> EEASSTGRNFNVE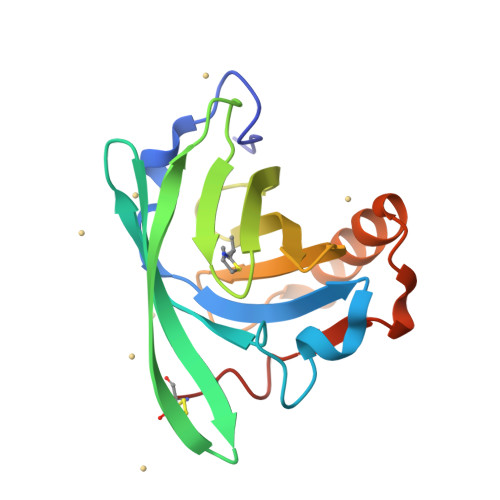KINGEWHTIILASDKREKIEDNGNFRLFLEQIHVLEKSLVLKFHTVRDEECSELSMVADKTEKAGEYSVTYDGFNTFTIPKTDYDNFLMAHLINEKDGETFQLMGLYGREPDLSSDIKERFAQLCEEHGILRENIIDLSNANRCLQARE>[3x]SRADDKGVMDYYLKYFSGAHDGDVYPAWSQKVEKKIRAKAFQ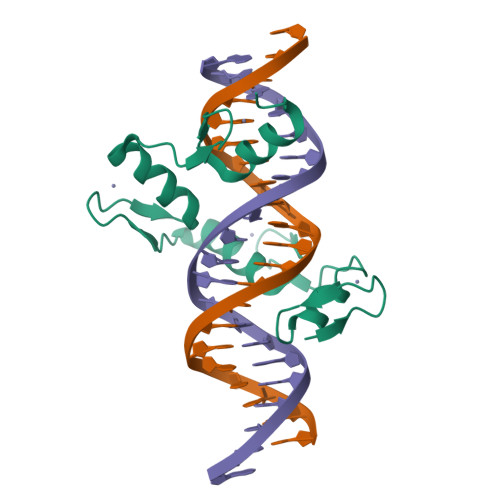KCPICEKVIQGAGKLPRHIRTHTGEKPYECNICKVRFTRQDKLKVHMRKHTGEKPYLCQQCGAAFAHNYDLKNHMRVHTGLRPYQCDSCCKTFVRSDHLHRHLKKDGCNGVPSRRGRKPRVRG> MRRNIFCLACLWIVQACLSLDRADILYNIRQTSRPDVIPTQ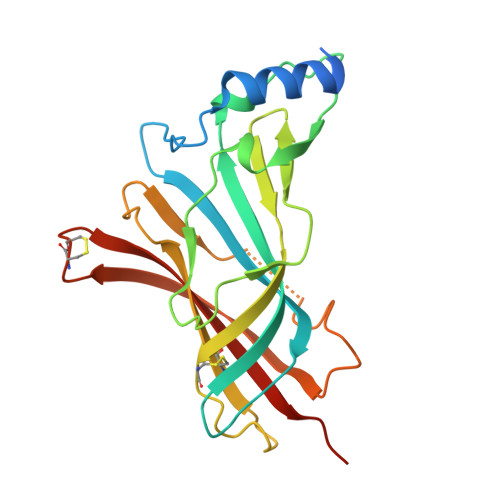RRPVAVSVSLKFINILEVNEITNEVDVVFWQQTTWSDRTLAWNSSHSPDQVSVPISSLWVPDLAAYNAISKPEVLTPQLAHVVSDGEVQYTPSIRQRFSCDVSGVDTESGATCRIKIGSWTHHSREISVDPTTENSDDSEYFSQYSRFEILDVTQKKNSVTYSCCPEAYEDVEVSLNFRKKGRSEIL>[3x]GQPVSALSILSLLERVSTIIDGVQASQQRMEERQQQLEGSVSAVQSELLKLAR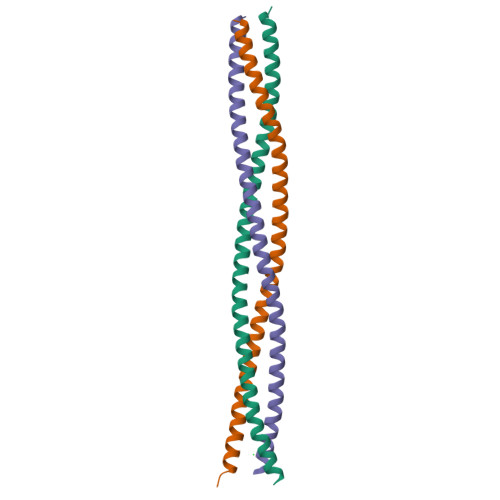DHGATATTVDKLLQKARRVSTHVKEVRSRVEKQNVRVKKVETTQDELLTRNKFRV>MSAQSLEVGQKARLSKRFGAAEVAAFAALSEDFNPLHLDPAFAATTAFERPIVHGMLLASLFSGLLGQQLPGKGSIYLGQSLSFKLPVFVGDEVTAEVEVTALREDKPIATLTTRIFTQGGALAVTGEAVVK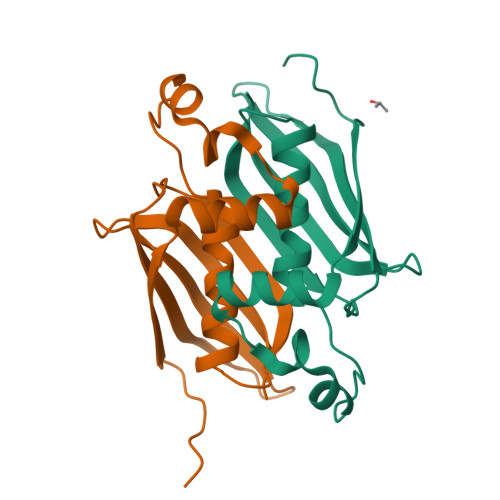LP[2x]>[3x]GPIGPPGPRGN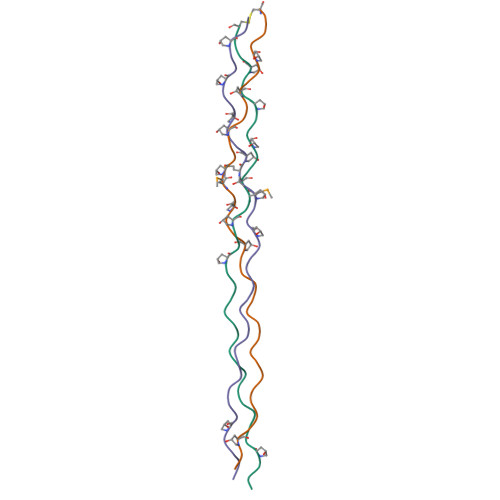RGERGSEGSPGHPGMPGPPGPPGAPGPCCGG> HIEGYECQPIFLNVLEAIEPGVVCAGHDNNQPDSFAALLSSLNELGERQLVHVVKWAKALPGFRNLHVDDQMAVIQYSWMGLMVFAMGWRSFTNVNSRMLYFAPDLVFNEYRMHKSRMYSQCVRMRHLSQEFGWLQITPQEFLCMKALLLFSIIPVDGLKNQKFFDELRMNYIKELDRIIACKRKNPTSCSRRFYQLTKLLDSVQPIARELHQFTFDLLIKSHMVSVDFPEMMAEIISVQ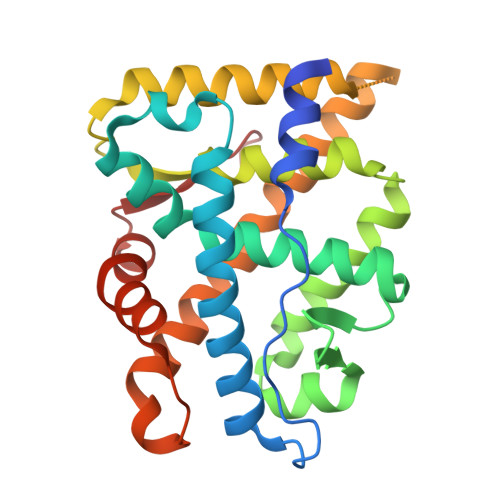VPKILSGKVKPIYFHTQ>[2x]GGGCCACUGUUCUCACUGU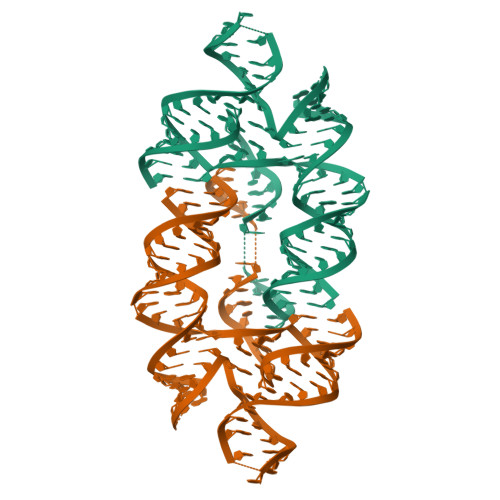UGCGCUACAUCUGGCUAUUCGGAAAUGGAAGCCAGACCACACGAAAGUGUGGAUUGACCAGUGGCCCCUCCCUGAAGGUAAACUUGUAGCGC> ASCTFTDAASAMASKTACSTITLNNIAVPAGTTLDLTGLTSGTRVIFEGTTTFGYQEWSGPLVSISGTDITVQGASGSVLDGDGARWWDGQGSNGGKTKPKFFYAHSLDSSSITGITIKNSPVQVFSIQSNNLSLTDITVDDADGDTQGGHNTDAFDIGSSTYITITNANVHNQDDCIAVNSGENIIFTGGTCTGGHGLSIGSVGGRSDNTVKNVTIEHSTVTNSQNGVRIKTVYGATGSVSEVTYSNIQMSGITNY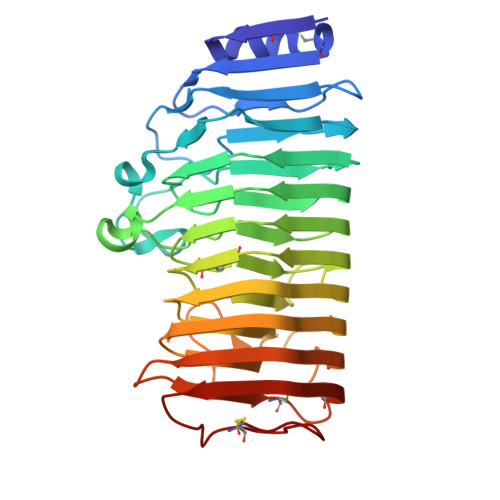GIVIEQDYENGSPTGTPTNGVPITDLTLNCVTGSVSSGATEIYILCGSGSCSSWTWTCVSITGGSKSTKCENVPSGVSC Here we elucidate the structural and molecular determinant(s) of target specificity of histidine vs. lysine in the active site of SETD3. On the substrate-binding surface, the residues are diverse, reflecting the fact that the three enzymes act on three very distinct substrates—the large subunit of Rubisco by LSMT, RelA subunit of nuclear factor NFκB by SETD6, and actin by SETD3—with limited sequence similarity immediately surrounding the methylation target. To facilitate the methyl transfer reaction, SETD3 provides a local environment that promotes deprotonation of the target nitrogen N3 of histidine (and concomitant protonation of N1). Most (if not all) SAM-dependent MTases use the classic SN2 reaction mechanism, which requires the target nitrogen be in a deprotonated state.

We hypothesized that the non-conserved Asn255 and its H-bond to the N1 atom of the imidazole ring is important for orienting and shifting the proton from N3-H to N1-H. Substituting Asn255 with alanine (N255A) or valine (N255V) resulted in reduced kcat values of 4.4 h−1 (N255A) or 1.3 h−1 (N255V) from 22 h−1 of wild-type (WT) SETD3, supporting the notion that kcat could be substantially slower if the substrate was a mix of the two protonation states. In addition, we determined the N255A mutant structures in complex with H73-containing and K73-containing peptides, respectively. Pairwise comparison between the WT and mutant enzyme complexed with the same peptide revealed identical overall structures with root-mean-square deviations of 0.4–0.5 Å across all Cα atoms. A small movement towards to the respective target residue (H73 or K73) is observed for Trp273 in the absence of side chain of Asn255. With no H-bond potential with the imidazole ring, N255A mutant reduced activity on H73 methylation, whereas the extra space generated by removing the side chain of N255 might provide flexibility for multiple round of K73 methylation (see below). In contrast, the activity on H73 is in the reverse order (WT≫N255A>N255V).

>[2x]GPLGSMGKKSRVKTQKSGTGATATVSPKEILNLTSELLQKCSSPAPGPGKEWEEYVQIRTLVEKIRKKQKGLSVTFDGKREDYFPDLMKWASENGASVEGFEMVNFKEEGFGLRATRDIKAEELFLWVPRKLLMTVESAKNSVLGPLYSQDRILQAMGNIALAFHLLCERASPNSFWQPYIQTLPSEYDTPLYFEEDEVRYLQSTQAIHDVFSQYKNTARQYAYFYKVIQTHPHANKLPLKDSFTYEDYRWAVSSVMTRQAQIPTEDGSRVTLALIPLWDMCNHTNGLITTGYNLEDDRCECVALQDFRAGEQIYIFYGTRSNAEFVIHSGFFFDNNSHDRVKIKLGVSKSDRLYAMKAEVLARAGIPTSSVFALHFTEPPISAQLLAFLRVFCMTEEELKEHLLGDSAIDRIFTLGNSEFPVSWDNEVKLWTFLEDRASLLLKTYKTTIEEDKSVLKNHDLSVRAKMAIKLRLGEKEILEKAVKSAAVNREYYRQQMEEKAPLPKYEESNLGLLESSVGDSRLPLVLRNLEEEAGVQDALNIREAISKAKATENGLVNGENSIPNGTRSENESLNQESKRAVEDAKGSSSDSTAGVKE;>[2x]TLKYPIEHGIVTNWD> GMGEKLELRLKSPVGAEPAVYPWPLPVYDKHHDAAHEI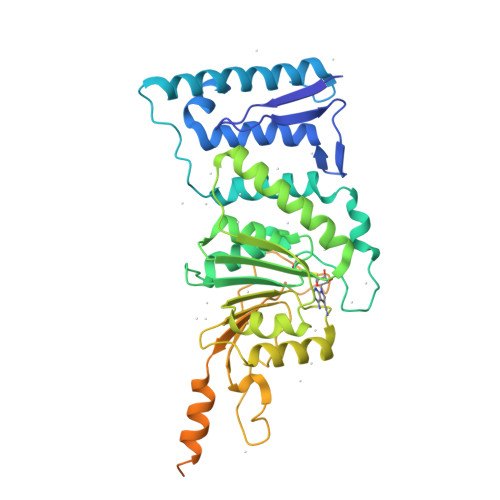IETIRWVCEEIPDLKLAMENYVLIDYDTKSFESMQRLCDKYNRAIDSIHQLWKGTTQPMKLNTRPSTGLLRHILQQVYNHSVTDPEKLNNYEPFSPEVYGETSFDLVAQMIDEIKMTDDDLFVDLGSGVGQVVLQVAAATNCKHHYGVEKADIPAKYAETMDREFRKWMKWYGKKHAEYTLERGDFLSEEWRERIANTSVIFVNNFAFGPEVDHQLKERFANMKEGGRIVSSKPFAPLNFRINSRNLSDIGTIMRVVELSPLKGSVSWTGKPVSYYLHTIDRTILENYFSSLKNPKLREEQEAARRRQQRESKSNAATPTKGPEGKVAGPADAPMDSGAEEEKAGAATVKKPSPSKARKKKLNKKGRKMAGRKRGRPKKMNTA>MQTSPAPAIVAGGAYQPVVLHAGIAY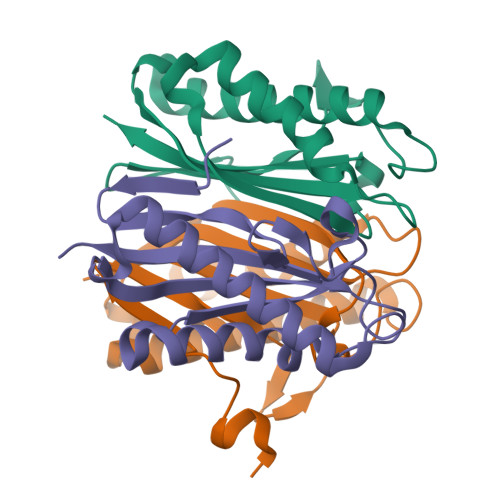VSGQLPRQHGELRWTGKVGSELDLEQARQAARLCAACCLLALEEALGGLQRVERLLKVTGYVASAAGFVQQPAVIDAASEYFDEVLGARGGHARAAVGVAELPRGAAVEVELIAAVRP[6x]>MPTVSQLQDGLEHPWSLAFLPAEQGLLITERPGRLRLWQQDKGLSPPIAGVPQVYAEGQGGLLEVLPAPDFAASRRVYLSFAEPGEGGKAGTAVGYGRLSDDDARLENFKVIFRQQPKLSVGNHFGGKLAFDRQGYLFIALGENNQRPTAQETDKLQGKLVRLTAEGAVPPDNPWVGQAGKRPEVWSYGHRNPQGLALNPWSGAIWEHEHGPRGGDELNIPLPGKNYGWPLATYGINYSGQPIPEAKGERVPGTEQPLHYWRVSPGLSGMAFYDGQRFPAWRHSLFIGALA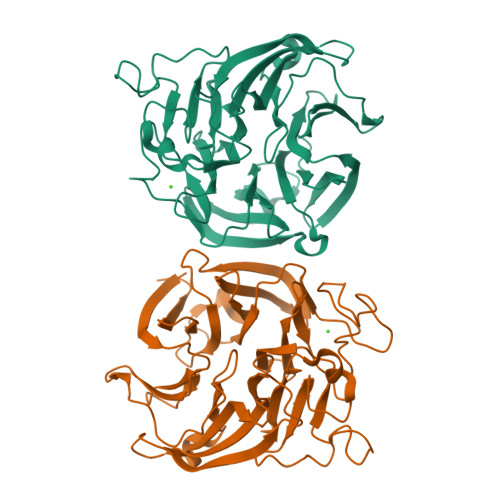QKALIRLTLEGDKVVAEERLLGDRGERIREVRSGPDGYLYLLTDERDGKLLKVGASLEHHHHHH[2x]> GIKVGVLGAKGRVGQTIVAAVNESDDLELVAEIGVDDDLSLLVDNGAEVVVDFTTPNAVMGNLEFCINNGISAVVGTTGFDDARLEQVRDWL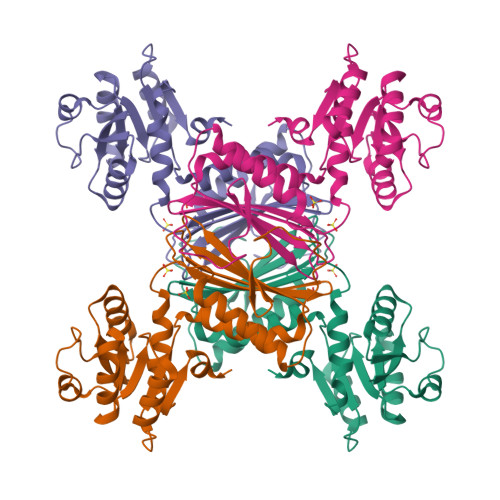EGKDNVGVLIAPNFAISAVLTMVFSKQAARFFESAEVIELHHPNKLDAPSGTAIHTAQGIAAARKEAGMDAQPDATEQALEGSRGASVDGIPVHAVRMSGMVAHEQVIFGTQGQTLTIKQDSYDRNSFAPGVLVGVRNIAQHPGLVVGLEHYLGL>[2x]DLYDDDDKDPTLMKISRGLLKTILEAAKSAHPDEFIALLSGSKDVMDELIFLPFVSGSVSAVIHLDMLPIGMKVFGTVHSHPSPSCRPSEEDLSLFTRFGKYHIIVCYPYDENSWKCYNRKGEEVELEVVEKD

The JAMM (JAB1/MPN/Mov34 metalloenzyme) motif in Rpn11 and Csn5 underlies isopeptidase activities intrinsic to the proteasome and signalosome, respectively. We show here that the archaebacterial protein AfJAMM possesses the key features of a zinc metalloprotease, yet with a distinct fold. In this study, we present the crystal structure of the Archaeoglobus fulgidus AF2198 gene product AfJAMM and explore the implications of its novel metalloprotease architecture. Unlike many JAMM proteins that contain an additional domain, the AfJAMM protein consists entirely of the JAMM domain.

AfJAMM consists of an eight-stranded β sheet (β1–β8), flanked by a long α helix (α1) between the first and second strand, and a short α helix (α2) between the fourth and fifth strand. The zinc-binding site is adjacent to a loop that spans the end of β4 to the beginning of α2 and is stabilized by a disulfide bond between C74 from this loop to C95 on β5. The overall fold resembles that of the zinc metalloenzyme cytidine deaminase (CDA). The two AfJAMM subunits in the asymmetric unit are connected through a parallel β sheet formed at the dimer interface. AfJAMM behaves as a monomer during size exclusion chromatography, suggesting that the dimer observed in the asymmetric unit is an artifact of crystallization. The zinc-binding site of AfJAMM is located in a furrow formed by the convex surface of the β2–β4 sheet and α2. The catalytic zinc has a tetrahedral coordination sphere, with ligands provided by Nɛ2 of H67 and H69 on β4, the carboxylate of D80 on α2, and a water molecule. The latter hydrogen-bonds to the sidechain of E22 on β2. Nonetheless, the active site metal and ligand atoms of thermolysin and ScNP can be superimposed on those of AfJAMM with an RMS deviation of approximately 0.4–0.5 Å. Meanwhile, the γ-hydroxyl group of the highly conserved S77 in AfJAMM occupies a position similar to Nɛ2 of H231 in thermolysin.SCLam, a GH16 member derived from a soil metagenome, an endo-β-1,3(4)-glucanase (EC 3.2.1.6), can cleave both β-1,3 and β-1,4 glycosidic bonds in glucans, such as laminarin, barley β-glucan, and cello-oligosaccharides. The enzyme SCLam has the typical β-jellyroll fold of GH16 family. The substrate-binding site is located on the concave face and is composed of the catalytic residues E144 and E149 (defined as nucleophile and acid/base, respectively) as well as other residues responsible for the substrate anchoring. All structures have a calcium-binding site with a Ca2+, heptacoordinated by a hydroxyl group from the E28, G72, and D258 main chain; D258 side chain; and three waters.

Although we did not manage to obtain the apo form of the mutated enzyme, the structures of SCLamE144S cocrystallized with five different substrates, BGB, BGC, C3, C6, and L6, were solved. It is surprising that, in all structures of enzyme-ligand complexes, except for SCLamE144S/L6, clear electron densities confirm the presence of a 1,3-β-D-cellobiosyl-glucose (G3), where the β-1,3 linkage is located at the reducing end, from subsite −3 to −1. In contrast, SCLamE144S/BGB and SCLamE144S/BGC do not have a clear electron density at positive subsites. Coincidentally, ITC curves from BGB and BGC were fitted to a single-site binding model. The SCLamE144S showed a 100-fold higher affinity to BGB than to BGC. This result is in contrast to the activity assays where the enzyme displays stronger preference for BGC over BGB. In summary, BGB may have high affinity to bind into negative subsites, thus preventing cleavage, whereas the BGC structure leads to optimal binding for hydrolysis. The presence of the same ligand (G3) in most structures, even when the enzyme was cocrystallized with cello-oligosaccharides, indicates a high affinity of G3 for this site. It is also noteworthy that all SCLamE144S structures have an α-anomeric glycan in subsite −1.

> GSHMQQPEGVTAPGNEPMAIPSDYKLVWADEFNTPGAPDAKKWRYDTSRNKEGWYNNELQYYAAGRPENVRVENGNLVIETRKERLTSMADYGGQEYSSGKLFTQGLADWQYGYVEVRAKLACGKGMWPAIWMMASDGSTGWPALGSIDIMEMVAWDPTTIHGTIHTKAYNHVIHTQKGSRTTAADPCGQFHTYSLDWTKDRMLIGVDGHAYMRFDNDHKGNHDTWPFDSPQYLILNVAIGGWGGQQGVDAAAFPSKMEVDYVRVYQKR>[4x]MASITDKDHQKVILVGDGAVGSSYAYAMVLQGIAQEIGIVDIFKDKTKGDAIDLSNALPFTSPKKIYSAEYSDAKDADLVVITAGAPQKPGETRLDLVNKNLKILKSIVDPIVDSGFNGIFLVAANPVDILTYATWKLSGFPKNRVVGSGTSLDTARFRQSIAEMVNVDARSVHAYIMGEHGDTEFPVWSHANIGGVTIAEWVKAHPEIKEDKLVKM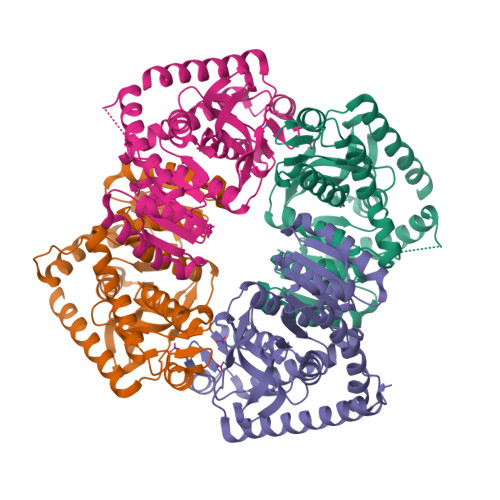FEDVRDAAYEIIKLKGATFYGIATALARISKAILNDENAVLPLSVYMDGQYGLNDIYIGTPAVINRNGIQNILEIPLTDHEEESMQKSASQLKKVLTDAFAKNDIETRQ>[2x]ASQFFFNQRTHLVSDVIDGAIIASPWNNLARLESDPAIRIVVRRDLNKNNVAVISGGGSGHEPAHVGFIGKGMLTAAVCGDVFASPSVDAVLTAIQAVTG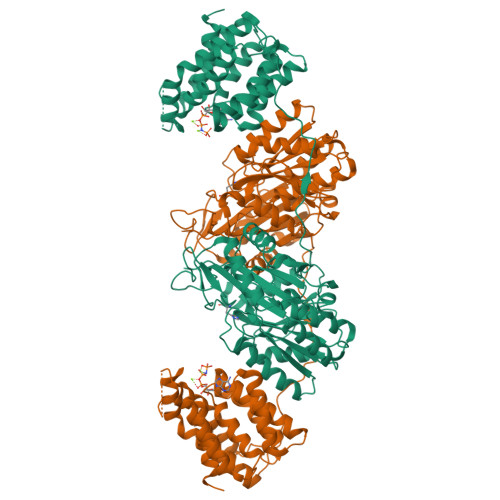EAGCLLIVKNYTGDRLNFGLAAEKARRLGYNVEMLIVGDDISLPDNKHPRGIAGTILVHKIAGYFAERGYNLATVLREAQYAASNTFSLGVALSSCHLPQETDAAPRHHPGHAELGMGIHGEPGASVIDTQNSAQVVNLMVDKLLAALPETGRLAVMINNLGGVSVAEMAIITRELASSPLHSRIDWLIGPASLVTALDMKGFSLTAIVLEESIEKALLTEVETSNWPTPVPPREITCVVSSHASARVEFQPSANALVAGIVELVTATLSDLETHLNALDAKVGDGDTGSTFAAAAREIASLLHRQQLPLNNLATLFALIGERLTVVMGGSSGVLMSIFFTAAGQKLEQGANVVEALNTGLAQMKFYGGADEGDRTMIDALQPALTSLLAQPKNLQAAFDAAQAGAERTCLSSKANAGRASYLSSESLLGNMDPGAQALAMVFKALAESELG>NAMIIRPEQHWFLRLFDWHGSVLSKIIFRLLLNVLMSIIAIISYQWYEQLGIHLTVAPFSLLGIAIAIFLGFRNSASYSRFVEARNLWGTVLIAERTLVRQLRNILPAEHDAHRRIVSYLVAFSWSLKHQLRKTDPTADLRRLLPEERVTEILASSMPTNRILLLAGNEIGQLREAGKLSDITYGLMDNKLDELAHVLGGCERLATTPVPFAATLILQRTVYLFCTLLPFALVGDLHYMTPFVSVFISYT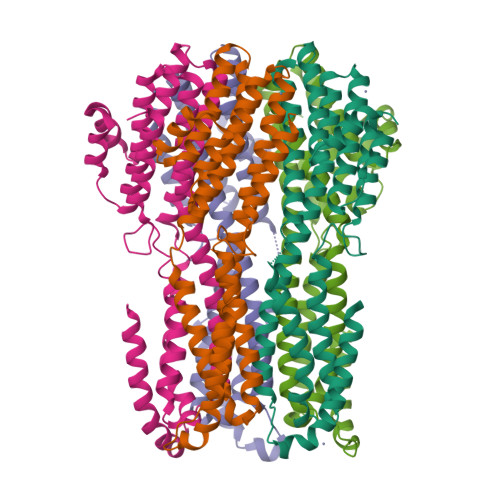FLSWDSLAEELEDPFGTAANDLPLNAMCNTIERNLLDMTGQHPLPE[5x]> MTGDHIKVIYFNGRGRAESILMTLVAAGVNYEDERISFQDWP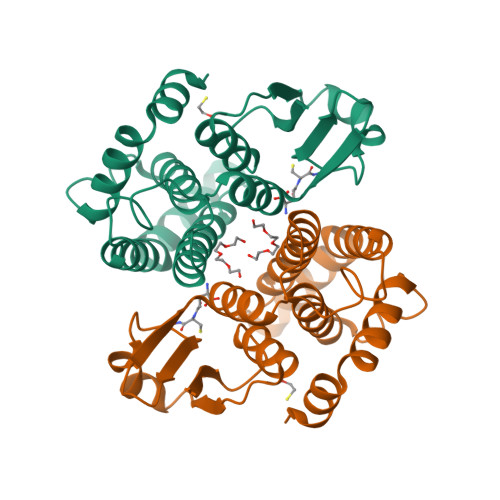KIKPTIPGGRLPAVKITDNHGHVKWMVESLAIARYMAKKHHMMGGTEEEYYNVEKLIGQAEDLEHEYYKTLMKPEEEKQKIIKEILNGKVPVLLDIICESLKASTGKLAVGDKVTLADLVLIAVIDHVTDLDKEFLTGKYPEIHKHRENLLASSPRLAKYLSDRAATPF> AGRKVVVVGGGTGGATAAKYIKLADPSIEVTLIEPNTDYYTCYLSNEVIGGDRKLESIKHGYDGLRAHGIQVVHDSATGIDPDKKLVKTAGGAEFGYDRCV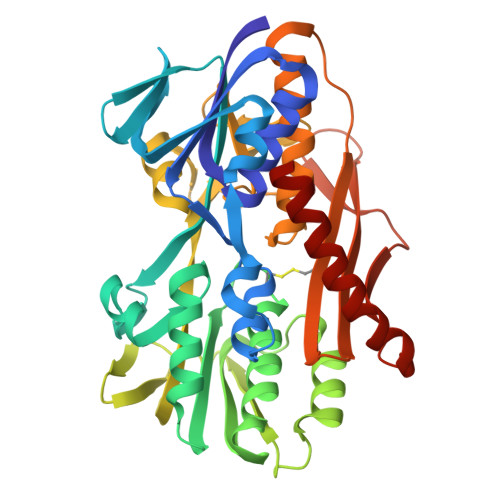VAPGIELIYDKIEGYSEEAAAKLPHAWKAGEQTAILRKQLEDMADGGTVVIAPPAAPFRCPPGPYERASQVAYYLKAHKPMSKVIILDSSQTFSKQSQFSKGWERLYGFGTENAMIEWHPGPDSAVVKVDGGEMMVETAFGDEFKADVINLIPPQRAGKIAQIAGLTNDAGWCPVDIKTFESSIHKGIHVIGDASIANPMPKSGYSANSQGKVAAAAVVVLLKGEEPGTPSYLNTCYSILAPAYGISVAAIYRPNADGSAIESVPDSGGVTPVDAPDWVLEREVQYAYSWYNNIVHDTFG>[2x]MRGSMANINDSKILSLQNRKNTLVDTSGYNAEVSEEGDVQLNPIFPFDFKLGSSGEDRGKVIVTQNENIVYNSMYESFSISFWIRINKWVSNLPGYTIIDSVKNNSGWSIGIISNFLVFTLKQNEDSEQSINFSYDISNNAPGYNKWFFVTVTNNMMGNMKIY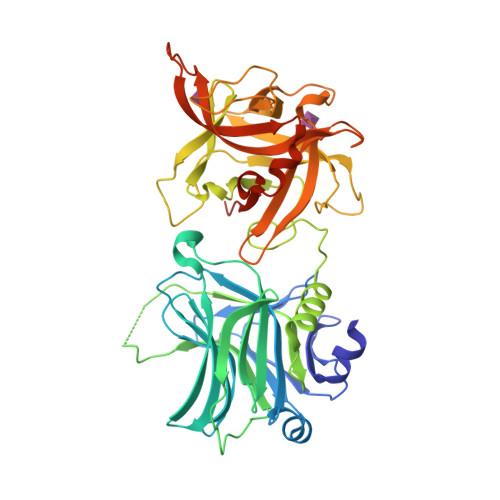INGKLIDTIKVKELTGINFSKTITFEINKIPDTGLITSDSDNINMWIRDFYIFAKELDGKDINILFNSLQYTNVVKDYWGNDLRYNKEYYMVNIDYLNRYMYANSRQIVFNTRRNNNDFNEGYKIIIKRIRGNTNDTRVRGGDILYFDMTINNKAYNLFMKNETMYADNHSTEDIYAIGLREQTKDINDNIIFQIQPMNNTYYYASQIFKSNFNGENISGICSIGTYRFRLGGDWYRHNYLVPTVKQGNYASLLESTSTHWGFVPVSEPGSAWSHPQFEK>MSELEKAMVALIDVFHQYSGREGDKHKLKKSELKELINN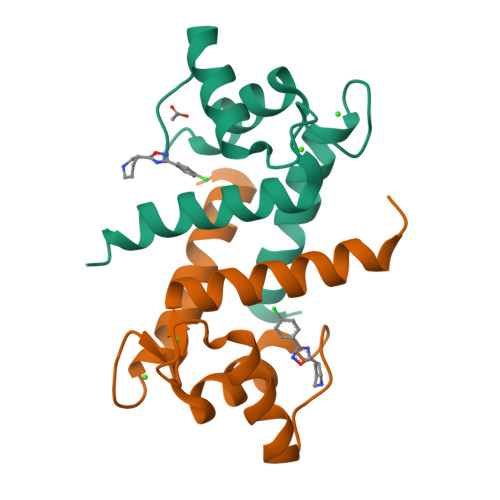ELSHFLEEIKEQEVVDKVMETLDNDGDGECDFQEFMAFVAMVTTACHEFFEHE[2x]>[2x]GPHMADPETAAKFKSKNAFPDPLNDPKCNPKSLVKKYLTPKVFESLKNKKTKLGITLWDCINSGVVNLDSGVGVYAGDEESYTLFGPLFDAIIEDYHSPYKLATGHNSDMNPAHVKAPDLDPANRYIRSTRIRVARSLKGYGLAPGVTKAHRLEIEKKVVGVLTSLTGDLAGKYYPLSGMDEKT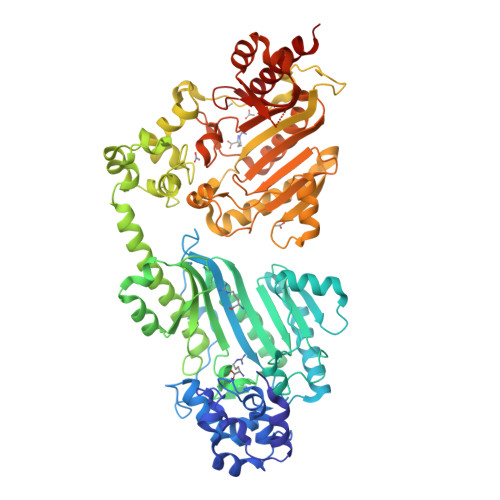RQQLVDDHFLFKKGDRFLEAAGINKEWPEGRGIYHNNDKTFLVWLNEEDHLRIISMEKGSDIGSVFSRLCRAVNEIDKKLGFQHTKKHGYLTSCPSNLGTGMRASVHVKIPHAKEHPDFENILTKYHIQARGIHGEHSESTGEDAGVYDISNRRRLGLSEVQCVQDMYDGVKALMELEKEAIAKKRSVFPEVLKNPEVKSLLRKYLTPELFDSLKDKKTAKGISLYDCINSGVENLDSSCGVYAGDEECYTLFAPLFDKIVEDYHSPYKLANKHTSDMNPEKVDAPNLDPEGTYIRSTRIRVARNVKGYALTPGLTRNERLDIERKVVGVLSSLTGDLAGQYYPLTGMDEATRQKLVNDHFLFKKGDRFLEAAGVNKLWPEGRGIFHNNDKTFLVWINEEDQLRIISMEKGSDIGSVFGRLCRAVNEIDKQLGFQHTDAHGYLSGCPTNLGTGMRASVHVKIPKASAHPDFQKICDEFHIQARGIHGEHSVSTGEDAGVFDISNRRRLGLSEVQCVQDMYNGVKKLLEIEKSTK> SDDT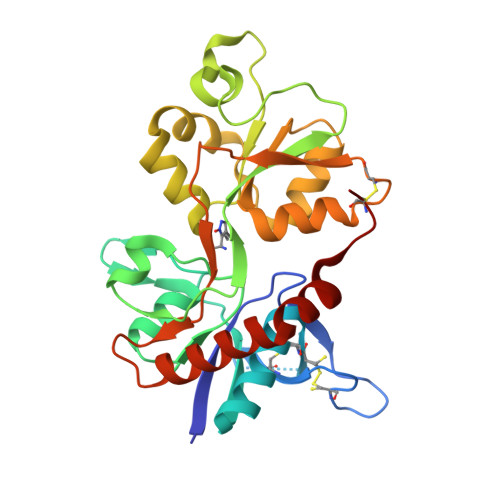QHLTVATLEERPFVIVEPADPISGTCIRDSVPCRSQLNRTHSPPPDAPRPEKRCCKGFCIDILKRLAHTIGFSYDLYLVTNGKHGKKIDGVWNGMIGEVFYQRADMAIGSLTINEERSEIVDFSVPFVETGISVMVARGTTVSGLSDRKFQRPQEQYPPLKFGTVPNGSTEKNIRSNYPDMHSYMVRYNQPRVEEALTQLKAGKLDAFIYDAAVLNYMARKDEGCKLVTIGSGKVFATTGYGIALHKGSRWKRPIDLALLQFLGDDEIEMLERLWLSGICHN N-[(2-chloro-6-fluorophenyl)methyl]-N,2-dimethylpyrimidine-4-carboxamide | C14 H13 Cl F N3 O | 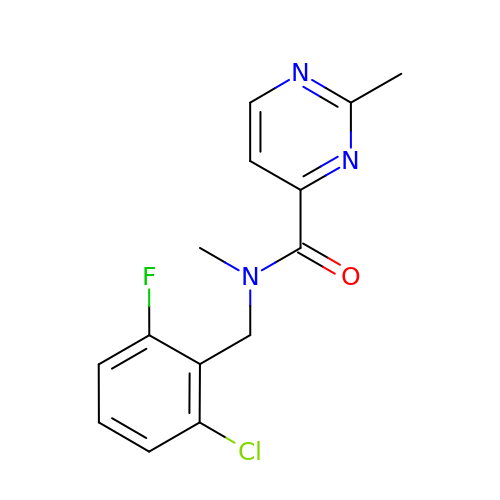MOTYBLMYPYOWBD-UHFFFAOYSA-N4-[5-(4-PHENOXYPHENYL)-1H-PYRAZOL-3-YL]MORPHOLINE | C19 H19 N3 O2 | 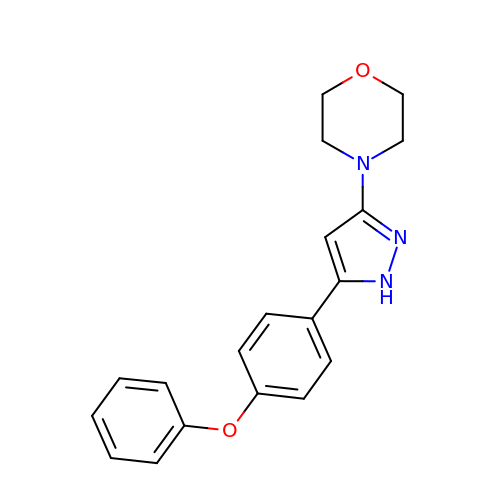WQWBZRVAFAMASC-UHFFFAOYSA-N> GSKQQTSALIHNIFDSHFAAIQIHHDSNSKSEVIRDF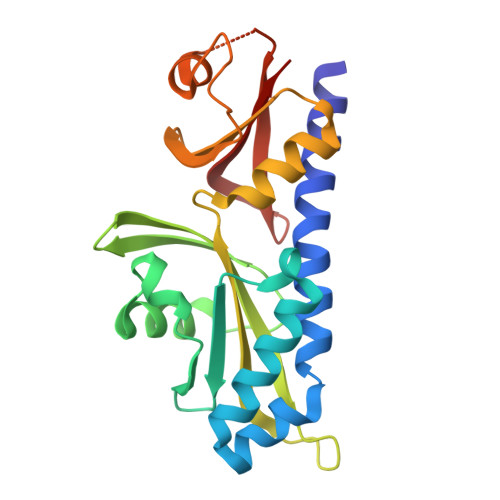YTDRDTDVLNFFFLSIDQSDPSHTPEFRFLTDHKGIIWDDGNAHFYGVNDLILDSLANRVSFSNNWYYINVMTSIGSRHMLVRRVPILDPSTGEVLGFSFNAVVLDNNFALMEKLKSESNVDNVVLVANSVPLANSLIGDEPYNVADVLQRKSSDKRLDKLLVIETPIVVNAVTTELCLLTVQD> MAHYPTRLKTRKTYSWVGRPLLDRKLHYQTYREMCVKTEGCSTEIHIQIGQFVLIEGDDDENPYVAKLLELFEDDSDPPPKKRARVQWFVRFCEVPACKRHLLGRKPGAQEIFWYDYPACDSNINAETIIGLVRVIPLAPKDVVPTNLKNEKTLFVKLSWNEKKFRPLSSELFAELNKPQESAAKCQKPVRAKSKSAESPSWTPAEHVAKRIESRHSASKSRQTPTHPLTPRARKRLELGNLGNPQMSQQTSCASLDSPGRIKRKVAFSEITSPSKRSQPDKLQTLSPALKAPEKTRETGLSYTEDDKKASPEHRIILRTRIAASKTIDIREERTLTPISGGQRSSVVPSVILKPENIKKRDAKEAKAQNEATSTPHRIRRKSSVLTMNRIRQQLRFLGNSKSDQEEKEILPAAEISDSSSDEEEASTPPLPRRAPRTVSRNLRSSLKSSLHTLTKVPKKSLKPRTPRCAAPQIRSRSLAAQEPASVLEEARLRLHVSAVPESLPCREQEFQDIYNFVESKLLDHTGGCMYISGVPGTGKTATVHEVIRCLQQAAQANDVPPFQYIEVNGMKLTEPHQVYVQILQKLTGQKATANHAAELLAKQFCTRGSPQETTVLLVDELDLLWTHKQDIMYNLFDWPTHKEARLVVLAIANTMDLPERIMMNRVSSRLGLTRMCFQPYTYSQLQQILRSRLKHLKAFEDDAIQLVARKVAALSGDARRCLDICRRATEICEFSQQKPDSPGLVTIAHSMEAVDEMFSSSYITAIKNSSVLEQSFLRAILAEFRRSGLEEATFQQIYSQHVALC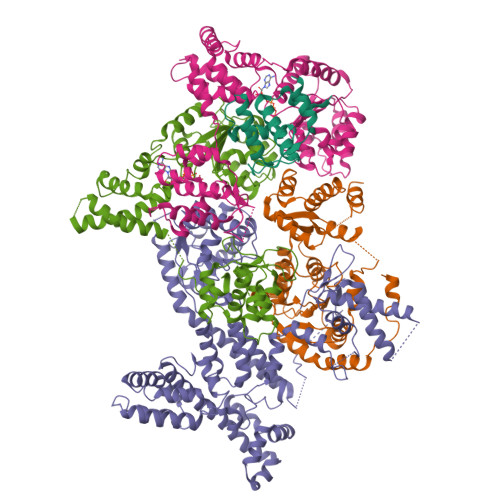RMEGLPYPTMSETMAVCSHLGSCRLLLVEPSRNDLLLRVRLNVSQDDVLYALKDE;> MSKPELKEDKMLEVHFVGDDDVLNHILDREGGAKLKKERAQLLVNPKKIIKKPEYDLEEDDQEVLKDQNYVEIMGRDVQESLKNGSATGGGNKVYSFQNRKHSEKMAKLASELAKTPQKSVSFSLKNDPEITINVPQSSKGHSASDKVQPKNNDKSEFLSTAPRSLRKRLIVPRSHSDSESEYSASNSEDDEGVAQEHEEDTNAVIFSQKIQAQNRVVSAPVGKETPSKRMKRDKTSDLVEEYFEAHSSSKVLTSDRTLQKLKRAKLDQQTLRNLLSKVSPSFSAELKQLNQQYEKLFHKWMLQLHLGFNIVLYGLGSKRDLLERFRTTMLQDSIHVVINGFFPGISVKSVLNSITEEVLDHMGTFRSILDQLDWIVNKFKEDSSLELFLLIHNLDSQMLRGEKSQQIIGQLSSLHNIYLIASIDHLNAPLMWDHAKQSLFNWLWYETTTYSPYTEETSYENSLLVKQSGSLPLSSLTHVLRSLTPNARGIFRLLIKYQLDNQDNPSYIGLSFQDFYQQCREAFLVNSDLTLRAQLTEFRDHKLIRTKKGTDGVEYLLIPVDNGTLTDFLEKEEEEA;> MATSSMSKGCFVFKPNSKKRKISLPIEDYFNKGKNEPEDSKLRFETYQLIWQQMKSENERLQEELNKNLFDNLIEFLQKSHSGFQKNSRDLGGQIKLREIPTAALVLGVNVTDHDLTFGSLTEALQNNVTPYVVSLQAKDCPDMKHFLQKLISQLMDCCVDIKSKEEESVHVTQRKTHYSMDSLSSWYMTVTQKTDPKMLSKKRTTSSQWQSPPVVVILKDMESFATKVLQDFIIISSQHLHEFPLILIFGIATSPIIIHRLLPHAVSSLLCIELFQSLSCKEHLTTVLDKLLLTTQFPFKINEKVLQVLTNIFLYHDFSVQNFIKGLQLSLLEHFYSQPLSVLCCNLPEAKRRINFLSNNQCENIRRLPSFRRYVEKQASEKQVALLTNERYLKEETQLLLENLHVYHMNYFLVLRCLHKFTSSLPKYPLGRQIRELYCTCLEKNIWDSEEYASVLQLLRMLAKDELMTILEKCFKVFKSYCENHLGSTAKRIEEFLAQFQSLDETKEEEDASGSQPKGLQKTDLYHLQKSLLEMKELRRSKKQTKFEVLRENVVNFIDCLVREYLLPPETQPLHEVVYFSAAHALREHLNAAPRIALHTALNNPYYYLKNEALKSEEGCIPNIAPDICIAYKLHLECSRLINLVDWSEAFATVVTAAEKMDANSATSEEMNEIIHARFIRAVSELELLGFIKPTKQKTDHVARLTWGGC;> MSSRKSKSNSLIHTECLSQVQRILRERFCRQSPHSNLFGVQVQYKHLSELLKRTALHGESNSVLIIGPRGSGKTMLINHALKELMEIEEVSENVLQVHLNGLLQINDKIALKEITRQLNLENVVGDKVFGSFAENLSFLLEALKKGDRTSSCPVIFILDEFDLFAHHKNQTLLYNLFDISQSAQTPIAVIGLTCRLDILELLEKRVKSRFSHRQIHLMNSFGFPQYVKIFKEQLSLPAEFPDKVFAEKWNENVQYLSEDRSVQEVLQKHFNISKNLRSLHMLLMLALNRVTASHPFMTAVDLMEASQLCSMDSKANIVHGLSVLEICLIIAMKHLNDIYEEEPFNFQMVYNEFQKFVQRKAHSVYNFEKPVVMKAFEHLQQLELIKPMERTSGNSEREYQLMKLLLDNTQIMNALQKYPNCPTDVRQWATSSLSWL;> MPHLENVVLCRESQVSILQSLFGERHHFSFPSIFIYGHTASGKTYVTQTLLKTLELPHVFVNCVECFTLRLLLEQILNKLNHLSSSEDGCSTEITCETFNDFVRLFKQVTTAENLKDQTVYIVLDKAEYLRDMEANLLPGFLRLQELADRNVTVLFLSEIVWEKFRPNTGCFEPFVLYFPDYSIGNLQKILSHDHPPEYSADFYAAYINILLGVFYTVCRDLKELRHLAVLNFPKYCEPVVKGEASERDTRKLWRNIEPHLKKAMQTVYLREISSSQWEKLQKDDTDPGQLKGLSAHTHVELPYYSKFILIAAYLASYNPARTDKRFFLKHHGKIKKTNFLKKHEKTSNHLLGPKPFPLDRLLAILYSIVDSRVAPTANIFSQITSLVTLQLLTLVGHDDQLDGPKYKCTVSLDFIRAIARTVNFDIIKYLYDFL>[2x]MKLKSLLLRYYPPGIMLEYEKHGELKTKSIDLLDLGPSTDVSALVEEIQKAEP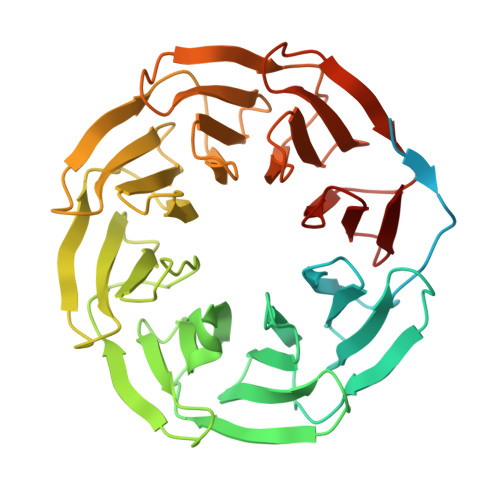LLTASRTEQVKLLIQRLQEKLGQNSNHTFYLFKVLKAHILPLTNVALNKSGSCFITGSYDRTCKLWDTASGEELNTLEGHRNVVYAIAFNNPYGDKIATGSFDKTCKLWSVETGKCYHTFRGHTAEIVCLSFNPQSTLVATGSMDTTAKLWDIQNGEEVYTLRGHSAEIISLSFNTSGDRIITGSFDHTVVVWDADTGRKVNILIGHCAEISSASFNWDCSLILTGSMDKTCKLWDATNGKCVATLTGHDDEILDSCFDYTGKLIATASADGTARIFSAATRKCIAKLEGHEGEISKISFNPQGNHLLTGSSDKTARIWDAQTGQCLQVLEGHTDEIFSCAFNYKGNIVITGSKDNTCRIWR>MGGSHHHHHHGDDDDKMTKTFKTLDDFLGTHFIYTYDNGWEYEWYAKNDHTVDYRIHGGMVAGQWVTDQKADIVMLTEGIYKISWTEPTGTDVALDFMPNEKKLHGTIFFP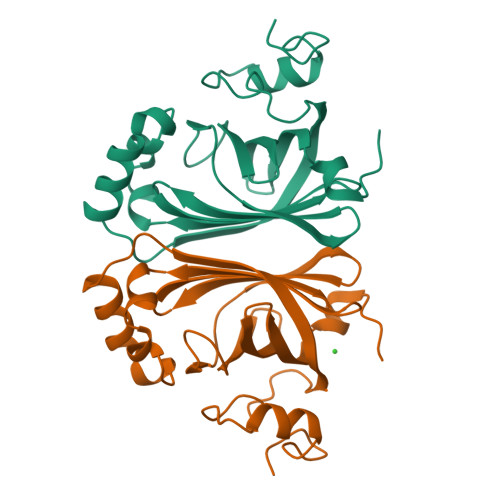KWVEEHPEITVTYQNEHIDLMEQSREKYATYPKLVVPEFANITYMGDAGQNNEDVISEAPYKEMPNDIRNGKYFDQNYHRLNK[4x]>TNIESKESFGKKVEDF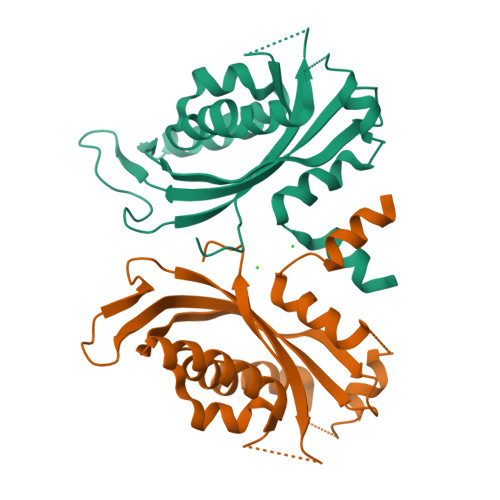KEKTVVGRSIQSLKNKLWDESENPLIVVMRKITNKVGGFFAETESSRVYSQFKLMDPTFSNESFTRHLREYIVPEILEAYVKGDVKVLKKWFSEAPFNVYAAQQKIFKEQDVYADGRILDIRGVEIVSAKLLAPQDIPVLVVGCRAQEINLYRKKKTGEIAAGDEANILMSSYAMVFTRDPEQIDDDETEGWKILEFVRGGSRQFT[2x]> EDPHLRNRPGKGHNY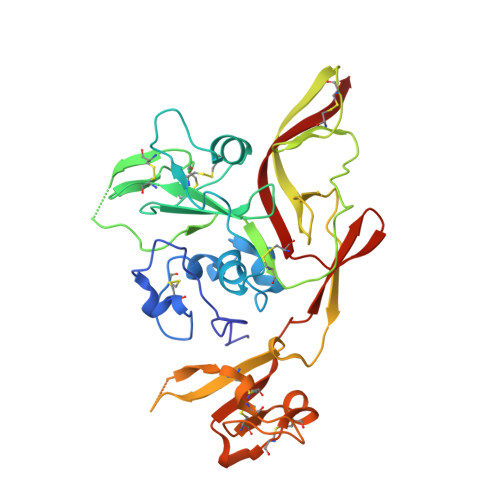IDGMTQEDATCKPVTYAGACSSFDVLLEKGKFPLFQSYAHHRTLLEAVHDTIIAKADPPSCDLQSAHGNPCMKEKLVMKTHCPNDYQSAHYLNNDGKMASVKCPPKYELTEDCNFCRQMTGASLKKGSYPLQDLFCQSSEDDGSKLKTKMKGVCEVGVQALKKCDGQLSTAHEVVPFAVFKNSKKVYLDKLDLKTEENLLPDSFVCFEHKGQYKGTMDSGQTKRELKSFDISQCPKIGGHGSKKCTGDAAFCSAYECTAQYANAYCSHANGSGIVQIQVSGVWKKPLCVGYERVVVKRELS> SNAMNKANLFIISAPSGAGKTSLVRALVKALAEIKISISHTTRPKRPGDQEGVDYFFIDETRFQAMVKEGAFLEHATIYERHYGTEKDWVLRQLKAGRDVLLEIDWQGARQIRELFPPALSIFILPPSIEALRERLIKRR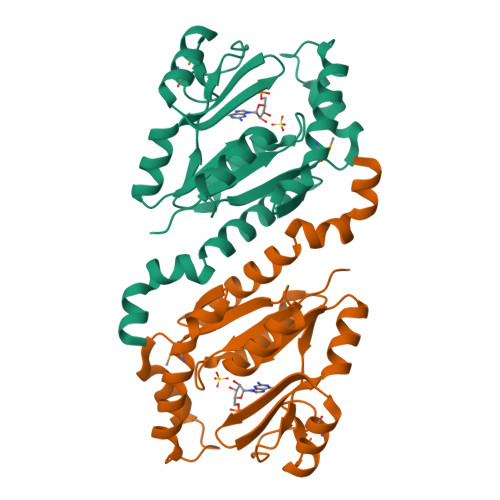QDDTAIIEQRLALAREEMAHYKEFDYLVVNDNFDQAVQNLIHIISAERLQRDVQEKKLSRLLAEL> GSFTGVIIKQGCLLKQGHRRKNWKVRKFILREDPAYLHYYDPAGAEDPLGAIHLRGCVVTSVESNSNGR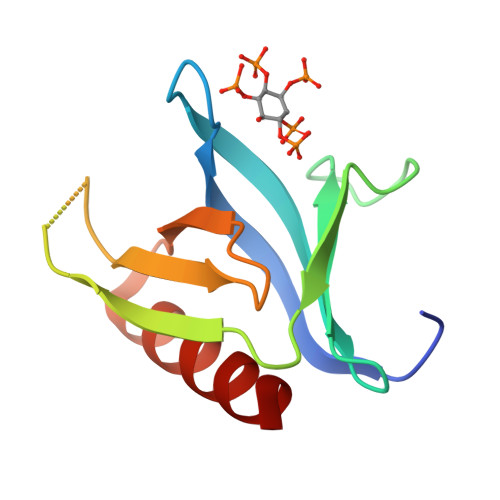KSEEENLFEIITADEVHYFLQAATPKERTEWIKAIQMASR>GPGSMVVARVYVGDVKEGQDRQWAVCVYCASGPTHPELLELAAEVGSSIAARGWTLVSGGGNVSAMGAVAQAARAKGGHTVGVIPKALVHRELADVDAAELIVTDTMRERKREMEHRSDAFIALPGGIGTLEEFFEAWTAGYLGMHDKPLILLDPFGHYDGLLTWLRGLVPTGYVSQRAMDSLVVVDNVEAALEAC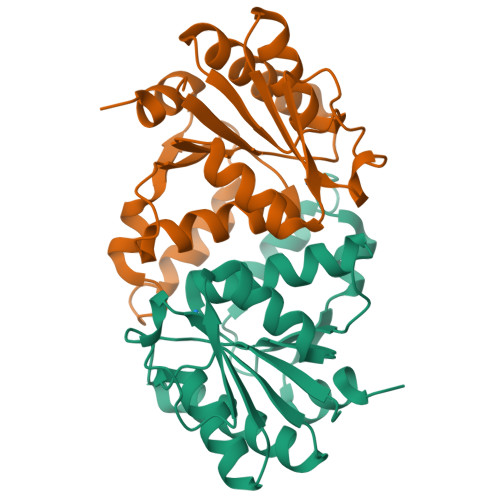APE[2x]N-(4-aminobutyl)-2-azidoacetamide | C6 H13 N5 O | 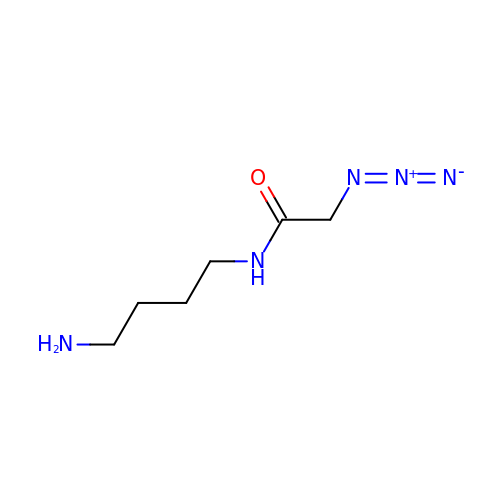SISZTIABCFMEIA-UHFFFAOYSA-N>MDDERKRKKYTLYLHPEKAADFQTLEAIESVPRSERGELFRNAFISGMALHQLDPRLPVLLTAILSEEFSADQVVTLLS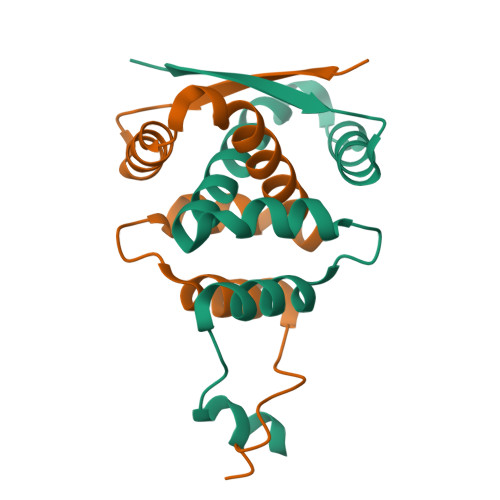QTTGWKPSQADIRAVLTELGASQSVEKMPPSATDSVQEAMNDVRLKMKKLF[2x]>MRGSHHHHHHGSPGLQEFMAATGANAEKAESHNDCPVRLLNPNIAKMKEDILYHFNLTTSRHNFPALFGDVKFVCVGGSPSRMKAFIRCVGAELGLDCPGRDYPNICAGTDRYAMYKVGPVLSVSHGMGIPSISIMLHELIKLLYYARCSNVTIIRIGTSGGIGLEPGTVVITEQAVDTCFKAEFEQIVLGKRVIRKTDLNKKLVQELLLCSAELSEFTTVVGNTMCTLDFYEGQGRLDGALCSYTEKDKQAYLEAAYAAGVRNIEMESSVFAAMCSACGLQAAVVCVTLLNRLEGDQISSPRNVLSEYQQRPQRLVSYFIKKKLSKA[4x]

Uridine phosphorylase (UPP; EC 2.4.2.3) is a ubiquitous enzyme that catalyzes the reversible phosphorolysis of uridine and analogous compounds to uracil and ribose-1-phosphate, playing an important role in pyrimidine salvage and regulation of uridine homeostasis. Interest in understanding the activity of human uridine phosphorylase (hUPP) stems from its role in the activation of pyrimidine nucleoside analogues used in chemotherapy, such as 5-fluorouracil (5-FU) and its prodrug, capecitabine. Most interestingly, the hexameric, trimer-of-dimers organization of prokaryotic UPPs has been dissociated in favour of strictly dimeric complexes in eukaryotic organisms. One of the unexpected findings of the first structures of hUPP1 was the discovery that the domains of the enzymatic dimer are flexibly linked, allowing an interdomain motion from an “open” ligand-free conformation to a “closed” catalytically-active structure.

Here we present the crystallographic structure of hUPP1 bound to 5-FU. The structure of hUPP1 bound to 5-FU provides further insight into this motion, having been crystallized in a transitional, intermediate position roughly 80% of the way from “open” to “closed”. Analysis of electron density distribution at the enzyme's active site reveals density in omit maps consistent with bound 5-FU. The fluorine moiety of 5-FU forms a hydrogen bond with Ser142 and is otherwise closely encased in a cluster of hydrophobic residues including Leu272, Leu273 and Ile281. Comparison of the architectures of BAU-bound and 5-FU bound monomers of hUPP1 reveals that substantial structural changes are restricted to a single loop region toward the back side of the active site. The 5-FU-bound structure shows that this conclusion is inaccurate, as the loop clearly closes around the small fluorine moiety of 5-FU. Specifically, in the BAU-bound structure of hUPP1, three partner-subunit residues assisted in the coordination, respectively, of the benzyl moiety (Tyr35), the ribose group (His36), and phosphate ion (Arg94). These chemical groups are all absent from the 5-FU-bound structure, eliminating every interdomain protein-ligand interaction. In spite of the lack of these stabilizing associations, all of these residues adopt conformations similar to those observed in the BAU-bound structure. Consistent with 5-FU not effectively stabilizing this interdomain conformation, the resulting structure is found partially open and the phosphate site unoccupied. Even a small obstruction that maintains the separation of Arg94 from Arg138 (as produced by crystal contacts in the 5-FU-bound structure) may effectively completely disrupt the enzyme's activity by preventing phosphate coordination and in turn, catalyzed phosphorolysis of uridine.> TNLSDIIEKETG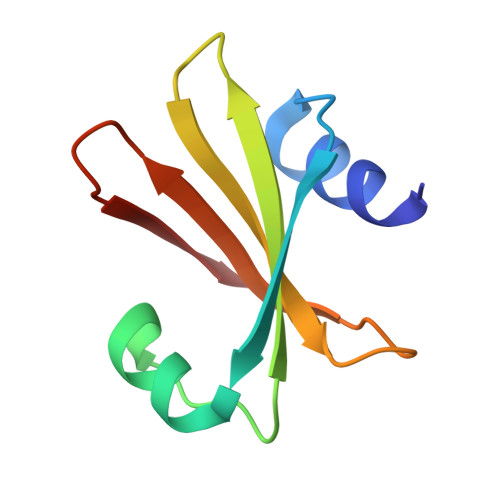KQLVIQESILMLPEEVEEVIGNKPESDILVHTAYDESTDENVMLLTSDAPEYKPWALVIQDSNGENKIKML>MEDYDVGGDMEWKRPSDPKFYITWATGKTFRVGDELEFDFAAGMHDVAVVTKDAFDNCKKENPISHMTTPPV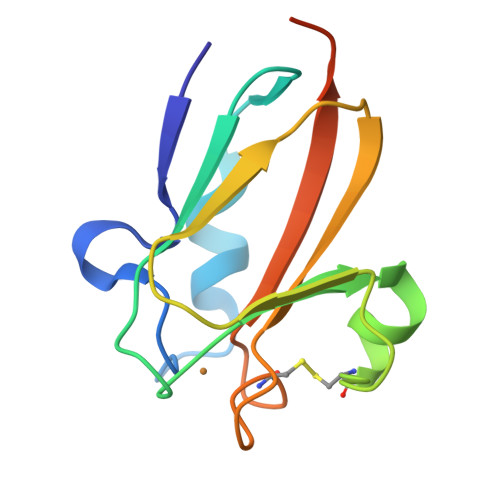KIMLNTTGPQYYICTVGDHCRVGQKLSINVVGAGGAGGGATPGA[2x]>MFEQRV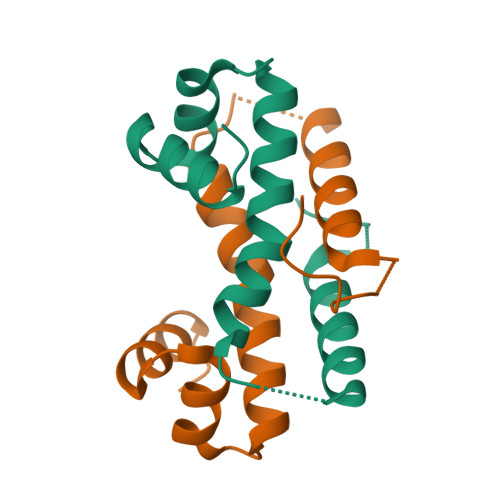NSDVLTVSTVNSQDQVTQKPLRDSVKQALKNYFAQLNGQDVNDLYELVLAEVEQPLLDMVMQYTRGNATRAALMMGINRGTLRKKLKKYGMN[2x]> GSRVALVTGANRGIGLAIARELCRQFSGDVVLTARDVA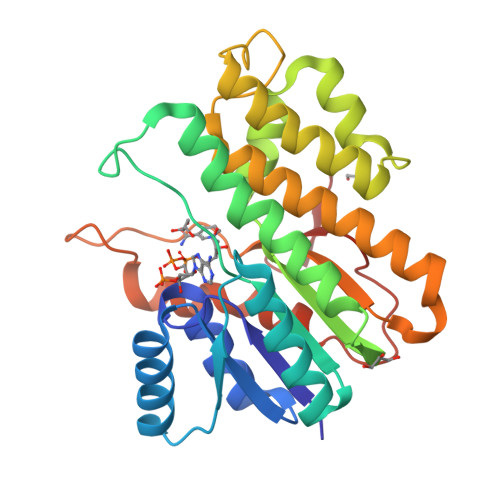RGQAAVQQLQAEGLSPRFHQLDIDDLQSIRALRDFLRKEYGGLNVLVNNAAVAFKSDDPMPFDIKAEMTLKTNFFATRNMCNELLPIMKPHGRVVNISSLQCLRAFENCSEDLQERFHSETLTEGDLVDLMKKFVEDTKNEVHEREGWPNSPYGVSKLGVTVLSRILARRLDEKRKADRILVNACCPGPVKTDMDGKDSIRTVEEGAETPVYLALLPPDATEPQGQLVHDKVVQNW>SNATKTIHNARYQALLDLLLEARSAAGITQKELAARLGRPQSFVSKTE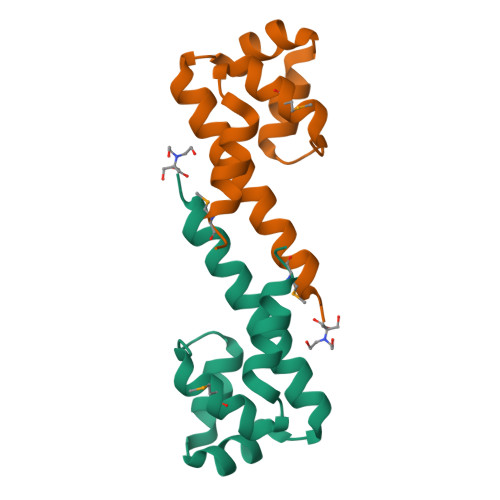NAERRLDVIEFMDFCRGIGTDPYALLSKLEAMTPS[5x]> NGIVPDAGHQGPDVSAVNGGTQVINIVTPNNEGISHNQYQDFNVGKPGAVFNNALEAGQSQLAGHLNANSNLNGQAASLILNEVVSRNPSFLLGQQEVFGIAAESVLSNPNGITCDGCG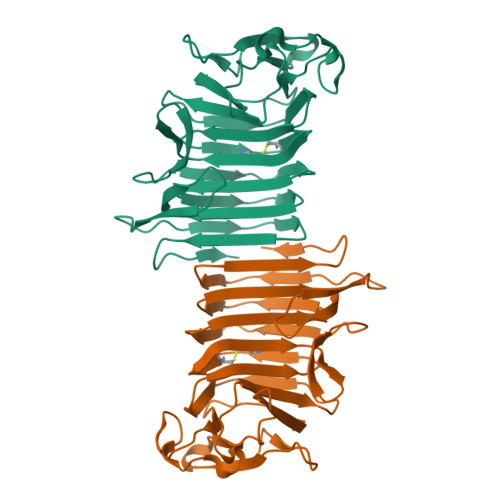FINTSRSSLVVGNPLFENGQLKGYSTLNNTNLLSLGKNGLNTTGLLDLIAPRIDSRGKITAAEISAFTGQNTFSQHFDILSSQKPVSALDSYFFGSMQSGRIRIINTAEGSGVKLAGHHHHHH> SYFQSNMLWALLRQYVRPYRWLLAVVAVLQVISNMASLYLPTVNAAIIDDGVAKGDTARIVELGAVMLGVTALQVVCAVGAVFFGARAATGFGHDLRAAVFTHVTTFSAEEAGRFGAASLLTRTTNDVGHIQQLVQLTVTMLITAPIMSIGGIFMALHQDAGLSWLLLVSVPVLGLANYWIIRHLMPVFTRMQSLIDGINRVLRDQLSGIRVIRAFAREPLERVRFAEANQTLSDSALEAGRWQALMLPVTTLVINVSSVALIWFGGLRIDAGQMQVGSLIAFLAYFMQILMAVLMATFMLVIFPRAAVCADRIGEVLSTQTAITNPADPVRPAAIAGDIGVHDATFCYPGADRPVLQDVSFTVPRGTTTAVVGSTGSGKSTLISLICRLYDVTSGSLRIDGVDVRDLDIEQLWSAIGLVPQR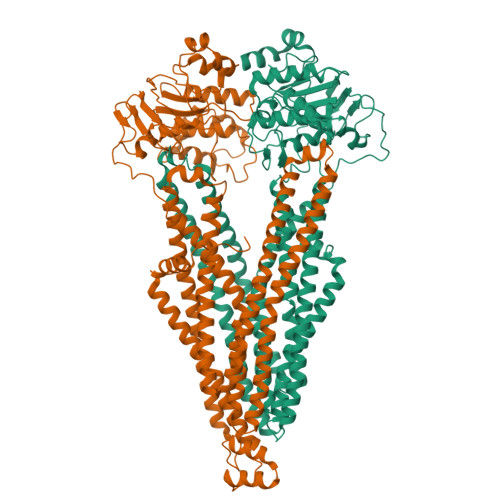GYLFSGTVAENLRYGRADATDDEMWEALRVAAAADFVRAHPQGLDMPVAQGGINFSGGQRQRLAIARAVIRRPAIYLFDDAFSALDVHTDARVRDALREVAADATVVIVSQRISTVIEADQVVVIDDGRVVGIGTHDTLLADCPIYAEFAESQALTAGEPR;> MRRGALPQAPLERTRDFKGSAIRLARRLLPQRALTLAVILLGVGGIAIGVIGPRILGHATDLLFNGVIGRELPAGLTKEQAVEAARARGDGTFADLLSGMDIVPGQGVDFGAVGRTLALALGLYLVAALLVWVQARLLNVTVQRTMVALRAEVQEKIHRLPLSYFDSRQRGEVLSRVTNDVDNIQNSVSMTISQLLTSVLTVFAVLVMMLTISPLLTLFTVVTVPASLWVTRWITRRSQPLFVAQWRNTGRLAAHLEETYSGFTIVKTFGHREAAAGKFAELNSETQQSSFGAQFFSGLVSPATMFIGNLSYVAVAVVGGLQVATGQITLGSIQAFIQYVRQFNQPLTQVAGMYNTLQSGIASAERVFDLLDTEEESADSPRRADVRTGRVEFEHVSFSYVPGTPVIEDLSLVAEPGSTVAIVGPTGAGKTTLVNLLMRFYDVDSGRITIDGVDIASVSRESLRASIGMVLQDTWLFAGTIYDNIAYGRPDADEDEVIEAATAAYVDRFVHTLPNGYDTRVDDDGGAISAGEKQLITIARAVLARPKLLVLDEATSSVDTRTELLIAHAMAELRRDRTSFIIAHRLSTIRDADLILVMDSGRIIERGTHEELLARHGRYWEMTRVHLGGIKAFHHHHHHHHHH> MELIRIAMRKDLENDKSLMSKWAAVAGLKNPNPLYDFLNHDGKTFSEFNSIVNIVKTHYPDQEYELMENYCLLLDPNTKAARSALEYADANSFNTLTDKLVEKMSIASNLKSKEYGKIYEIHRKLSRGEIDVLEASKNIGKYRIKTDEMNIFSKMIPMYDYLSKGNFSPMKSLLKQIDLNDIKENNYLKKSFETRIYVLLSNIYLNENELELSRKYAEKAIKSTDTKRFLVFSYLTIGTSYIFSDYALSKQNYLSGYEIAKGNSVFEEFFKRNLSFLNNFWNKENPWINYDSNAVTDVQEVIFELINQKKLERALTLLKSLERKKQNENDLGFHYYLEGLITNDKEAFYKSVEYFKL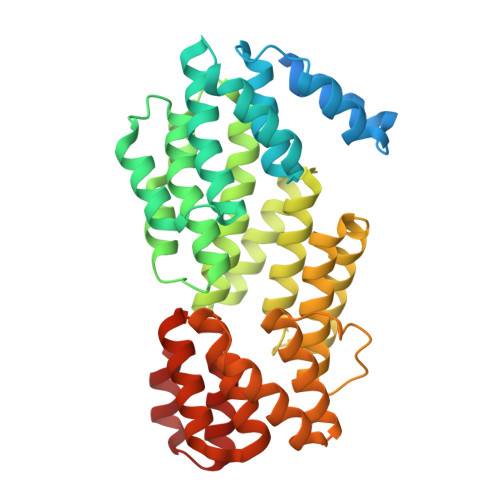SQDKLFIKMPLIKLESLGENPRLLKIISM(4-amino-1,2,5-oxadiazol-3-yl)[(3R)-3-{4-[(3-methoxyphenyl)amino]-6-methylpyridin-2-yl}pyrrolidin-1-yl]methanone | C20 H22 N6 O3 | 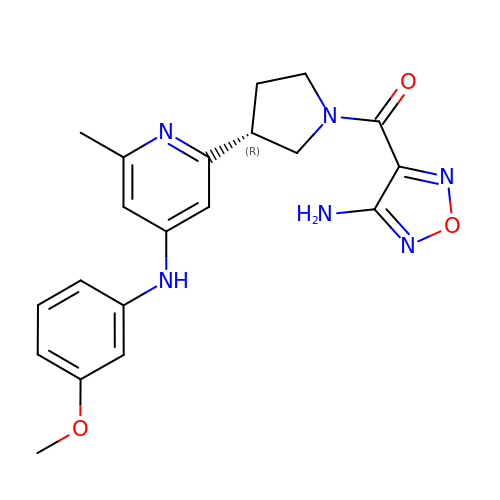BJUGLSYIEXNITK-CYBMUJFWSA-N> MKNILRLTLNGRAREDLVPDNMLLLDYLRETVGLTGTKQGCDGGECGACTVLVDDRPRLACSTLAHQVAGKKVETVESLATQGTLSKLQAAFHEKLGTQCGFCTPGMIMASEALLRKNP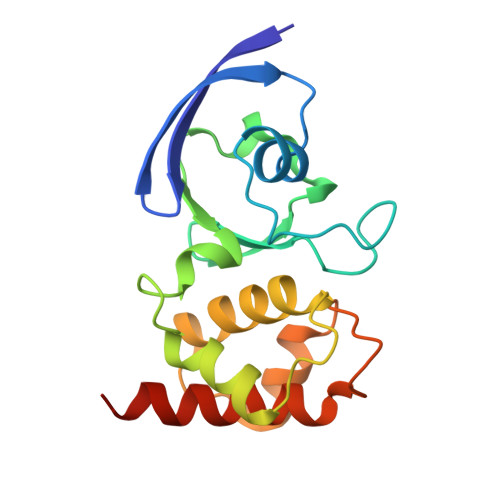SPSRDEIKAALAGNLCRCTGYVKIIKSVETAAAARLCEEGAR> PNAAATQVDGTQMSLLSVPEETSPAVEALENLDPRSLTPRQALEWIYRLKS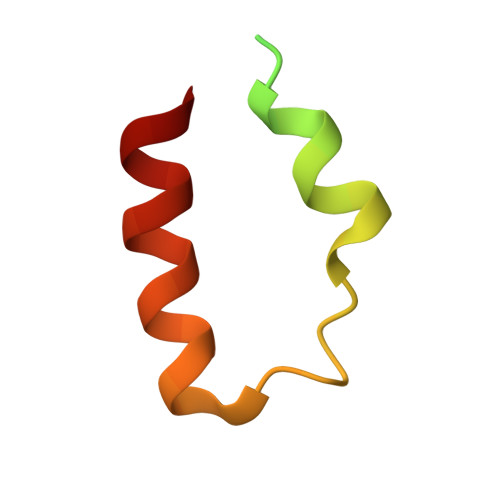LV[2-methyl-3-oxidanyl-5-(phosphonooxymethyl)pyridin-4-yl]methyl-(3-oxidanyl-1,2-oxazol-4-yl)azanium 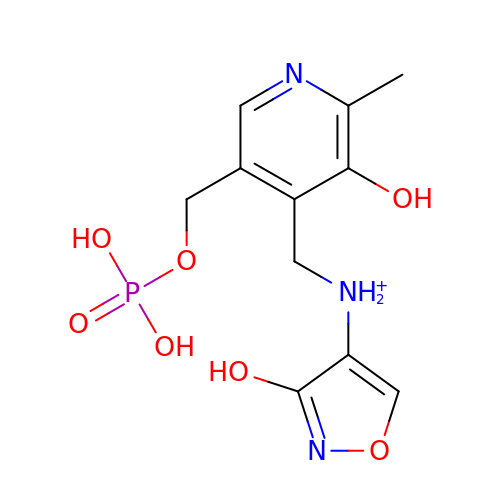| C11 H15 N3 O7 P | PXWFNGNWQUPGPJ-UHFFFAOYSA-O> MSLSPLAKEFLDEIERIQAEVAKNGREAVAEKYAPKSLEDNEENREAAYRFLLVNFPDDFSEEDKKLLEDFFKWFSEHFPEEFLKDLIYDTAFAAYVEAKKQGDPTLVLPITLYAAFLAFLEEWKKKYPESLTPELKELIEKLKELLEEAEKNDPRYKQAQAPIAAAKEAAKKQFKKYTSGSGHHHHHH

Here we use a robust deep learning pipeline to design complex folds and soluble analogues of integral membrane proteins. Unique membrane topologies, such as those from G-protein-coupled receptors, are not found in the soluble proteome, and we demonstrate that their structural features can be recapitulated in solution. Biophysical analyses demonstrate the high thermal stability of the designs, and experimental structures show remarkable design accuracy. The soluble analogues were functionalized with native structural motifs, as a proof of concept for bringing membrane protein functions to the soluble proteome, potentially enabling new approaches in drug discovery.

Next, we attempted to design a larger fold and a more intricate topology, the rhomboid protease fold (RPF). In addition, it harbours a serine–histidine catalytic dyad buried in the cell membrane, allowing it to cleave transmembrane protein domains and play an important part in cell signalling, which makes it a therapeutically interesting target. We selected 15 designs for protein expression, of which 13 were found to be soluble and five were selected for further experimental characterization. Three of the five designs showed a single monomeric species in solution and the expected helical secondary structure as assessed by circular dichroism. All of the three monomeric species of RPFs exhibited high thermal stability, with Tm above 90 °C. Notably, the AF2 structure predictions for the designs were less accurate than those for the CLF designs, with the r.m.s.d.Cα values between models and predictions ranging from 3.34 to 5.57 Å. In the case of the rhomboid protease design RPF_9, we observed high accuracy between the X-ray structure and the design model, with r.m.s.d.Cα of 0.97 Å and r.m.s.d.fa of 1.83 Å. However, the structural similarity was significantly lower compared with the target fold, as indicated by an r.m.s.d.Cα of 5.67 Å. Specifically, large structural deviations in the first extracellular loop were observed, which could have been due to its native positioning in the water–membrane interface. The designed RPF_9 fold showed significantly increased hydrophobicity on the transmembrane surface compared with the native RPF fold.> GDVQNAVEGAMVRVADTVQTSATNSERVPNLTAVETGHTSQAVPGDTMQTRHVINNHVRSESTIENFLARSACVFYLEYKTGTKEDSNSFNNWVITTRRVAQLRRKLEMFTYLRFDMEITVVITSSQDQSTSQNQNAPVLTHQIMYVPPGGPIPVSVDDYSWQTSTNPSIFWTEGNAPARMSIPFISIGNAYSNFYDGWSHFSQAGVYGFTTLNNMGQLFFRHVNKPNPAAITSVARIYFKPKHVRAWVPRPPRLCPYINSTNVNFEPKPVTEVRTNIITT;> SPTVEECGYSDRVRSITLGNSTITTQECANVVVGYGEWPEYLSDNEATAEDQPTQPDVATCRFYTLDSVQWEN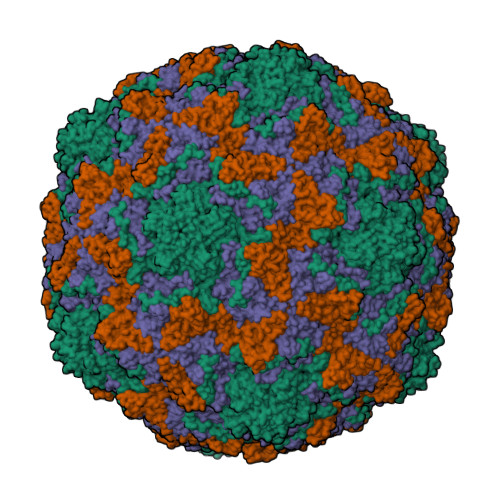GSPGWWWKFPDALRDMGLFGQNMYYHYLGRAGYTIHVQCNASKFHQGCILVVCVPEAEMGSAQTSGVVNYEHISKGEIASRFTTTTTAEDHGVQAAVWNAGMGVGVGNLTIFPHQWINLRTNNSATIVMPYVNSVPMDNMYRHHNFTLMIIPFVPLDFSAGASTYVPITVTVAPMCAEYNGLRLAGHQ;> GLPTMNTPGSNQFLTSDDFQSPSAMPQFDVTPEMHIPGEVRNLMEIAEVDSVMPINNDSAAKVSSMEAYRVELSTNTNAGTQVFGFQLNPGAESVMNRTLMGEILNYYAHWSGSIKITFVFCGSAMTTGKFLLSYAPPGAGAPKTRKDAMLGTHVVWDVGLQSSCVLCIPWISQTHYRFVEKDPYTNAGFVTCWYQTSVVSPASNQPKCYMMCMVSACNDFSVRMLRDTKFIEQTSFYQ;> GAQVSTQKTGAHETSLSATGNSIIHYTNINYYKDAASNSANRQDFTQDPGKFTEPMKDVMIKTLPALN> SKYVDRVIAEVEKKYADEPEFVQTVEEVLSSLGPVVDAHPEYEEVALLERMVIPERVIEFRVPWEDDNGKVHVNTGYRVQFNGAIGPYLGGLRFAPSVNLSIMKFLGFEQAFKDSLTTLPM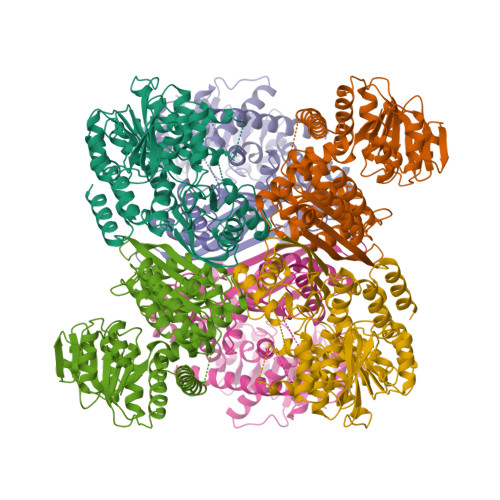GGAKGGSDFDPNGKSDREVMRFCQAFMTELYRHIGPDIDVPAGDLGVGAREIGYMYGQYRKIVGGFYNGVLTGKARSFGGSLVRPEATGYGSVYYVEAVMKHENDTLVGKTVALAGFGNVAWGAAKKLAELGAKAVTLSGPDGYIYDPEGITTEEKINYMLEMRASGRNKVQDYADKFGVQFFPGEKPWGQKVDIIMPCATQNDVDLEQAKKIVANNVKYYIEVANMPTTNEALRFLMQQPNMVVAPSKAVNAGGVLVVGFEMSQNSERLSWTAEEVDSKLHQVMTDIHDGSAAAAERYGLGYNLVAGANIVGFQKIADAMMAQGIAW> AGMSLTQVSGPVYVVEDNYYVQENSMVYFGAKGVTVVGATWTPDTARELHKLIKRVSRKPVLEVINTNYHTDRAGGNAYWKSIGAKVVSTRQTRDLMKSDWAEIVAFTRKGLPEYPDLPLVLPNVVHDGDFTLQEGKVRAFYAGPAHTPDGIFVYFPDEQVLYGNCILKEKLGNLSFADV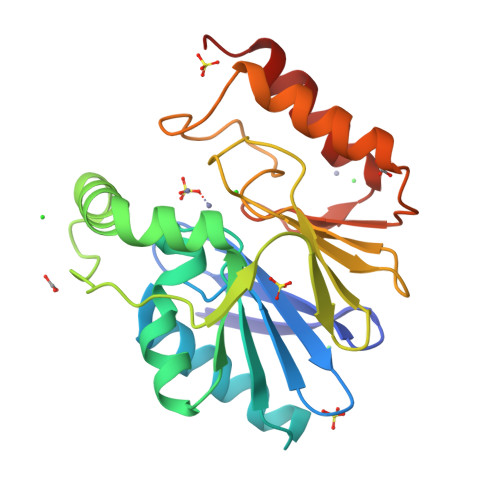KAYPQTLERLKAMKLPIKTVIGGHDSPLHGPELIDHYEALIKAAPQS> GRPILEVPESVTGPWKGDVNLPCTYDPLQGYTQVLVKWLVQRGSDPVTIFLRDSSGDHIQQAKYQGRLHVSHKVPGDVSLQL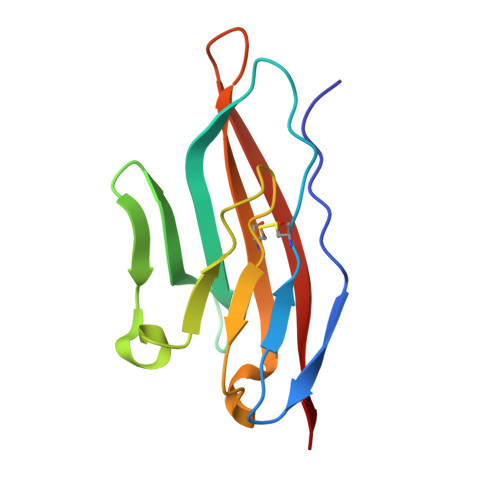STLEMDDRSHYTCEVTWQTPDGNQVVRDKITELRVQK Isocitrate dehydrogenases (IDHs) are the enzymes that catalyze the oxidative decarboxylation of isocitrate (ICT) into α-ketoglutarate (α-KG) and CO2 while converting the coenzyme NAD+ or NADP+ into NADH or NADPH. Mammalian NAD-IDH functions as a heterotetramer consisting of two α subunits (37 kDa), one β subunit (39 kDa), and one γ subunit (39 kDa). Previous biochemical studies have shown that the enzymatic activity of mammalian NAD-IDH could be positively regulated by citrate (CIT) and ADP; and in the α2βγ heterotetramer, the α subunit exerts the catalytic role, and the β and γ subunits play the regulatory roles. In this work, we examined the inhibition of the αβ and αγ heterodimers and the α2βγ heterotetramer of human NAD-IDH by NADH and found that all these enzymes can be substantially inhibited by NADH.

To understand the inhibitory mechanism of the αγ heterodimer by NADH, we solved the crystal structure of the αγ heterodimer bound with an Mg2+ and an NADH at the active site and an NADH at the allosteric site (αMg+NADHγNADH) at 2.4 Å resolution using the molecular replacement method. The structure belongs to space group P3121 containing one αγ heterodimer per asymmetric unit. The overall structure of the αMg+NADHγNADH heterodimer resembles that of the αMgγ heterodimer, representing the inactive state of the enzyme. In the αMg+NADHγNADH structure, the NAD+-binding site is bound with an NADH: the adenine moiety of the NADH is located at the deep pocket of the active site and the nicotinamide moiety positioned in close to the ICT-binding site. The NADH makes hydrogen-bonding interactions with a number of residues from the large domain of the α subunit, including Lys69A, Thr74A, Asn84A, Glu260A, His263A, Gly264A, Thr265A, Asp268A, and Asn276A. Surprisingly, in the αMg+NADHγNADH structure, there is an NADH bound at the allosteric site, which occupies a large portion of the allosteric site. Compared with the αMgγMg+CIT+ADP structure, the ADP moiety and nicotinamide-ribose moiety of NADH occupy fully the ADP-binding site and the nicotinamide moiety of NADH occupies the Mg2+-binding site and part of the CIT-binding site, making extensive hydrophilic and hydrophobic interactions with the surrounding residues. Particularly, in the αMg+NADHγNADH structure, the hydrogen-bonding interactions between the side chains of Arg97G and Tyr135G and between the side chains of Asn78G and Arg272G at the allosteric site are retained, and thus all the side chains of these residues are oriented outwards from the CIT-binding site. In addition, the N-terminal regions of the α7A and α7G helices at the heterodimer interface assume loop conformation instead of helical conformation, and make no hydrogen-bonding interactions with the β7A and β7G strands of the clasp β-sheet.

> TGGVQTVTLIPGDGIGPEISAAVMKIFDAAKAPIQWEERNVTAIQGPGGKWMIPSEAKESMDKNKMGLKGPLKTPIAAGHPSMNLLLRKTFDLYANVRPCVSIEGYKTPYTDVNIVTIRENTEGEYSGIEHVIVDGVVQSIKLITEGASKRIAEFAFEYARNNHRSNVTAVHKANIMRMSDGLFLQKCREVAESCKDIKFNEMYLDTVCLNMVQDPSQFDVLVMPNLYGDILSDLCAGLIGGLGVTPSGNIGANGVAIFESVHGTAPDIAGKDMANPTALLLSAVMMLRHMGLFDHAARIEAACFATIKDGKSLTKDLGGNAKCSDFTEEICRRVKDLD;> FSEQTIPPSAKYGGRHTVTMIPGDGIGPELMLHVKSVFRHACVPVDFEEVHVSSNADEEDIRNAIMAIRRNRVALKGNIETNHNLPPSHKSRNNILRTSLDLYANVIHCKSLPGVVTRHKDIDILIVRENTEGEYSSLEHESVAGVVESLKIITKAKSLRIAEYAFKLAQESGRKKVTAVHKANIMKLGDGLFLQCCREVAARYPQITFENMIVDNTTMQLVSRPQQFDVMVMPNLYGNIVNNVCAGLVGGPGLVAGANYGHVYAVFETATRNTGKSIANKNIANPTATLLASCMMLDHLKLHSYATSIRKAVLASMDNENMHTPDIGGQGTTSEAIQDVIRHIRVINGRAVEA>[4x]MTSASSPPAFRLETSDGDEEGNAEVNKGKQEPPPMESPFQREDRNSSPQIKVNLNFIKRPPKNTSAPSQQEPDRFDRDRLFSVVSRGVPEELTGLLEYLRWNSKYLTDSAYTEGSTGK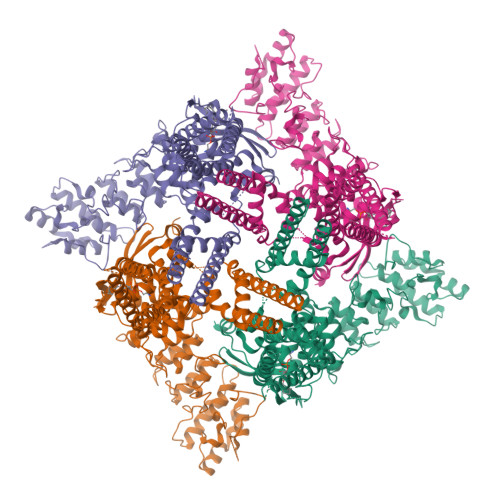TCLMKAVLNLQDGVNACIMPLLQIDKDSGNPKLLVNAQCTDEFYQGHSALHIAIEKRSLQCVKLLVENGADVHLRACGRFFQKHQGTCFYFGELPLSLAACTKQWDVVTYLLENPHQPASLEATDSLGNTVLHALVMIADNSPENSALVIHMYDGLLQMGARLCPTVQLEEISNHQGLTPLKLAAKEGKIEIFRHILQREFSGPYQPLSRKFTEWCYGPVRVSLYDLSSVDSWEKNSVLEIIAFHCKSPNRHRMVVLEPLNKLLQEKWDRLVSRFFFNFACYLVYMFIFTVVAYHQPSLDQPAIPSSKATFGESMLLLGHILILLGGIYLLLGQLWYFWRRRLFIWISFMDSYFEILFLLQALLTVLSQVLRFMETEWYLPLLVLSLVLGWLNLLYYTRGFQHTGIYSVMIQKVILRDLLRFLLVYLVFLFGFAVALVSLSREARSPKAPEDNNSTVTEQPTVGQEEEPAPYRSILDASLELFKFTIGMGELAFQEQLRFRGVVLLLLLAYVLLTYVLLLNMLIALMSETVNHVADNSWSIWKLQKAISVLEMENGYWWCRRKKHREGRLLKVGTRGDGTPDERWCFRVEEVNWAAWEKTLPTLSEDPSGPGITGNKKNPTSKPGKNSASEEDHLPLQVLQSP>MSLRPCFVSLIDESDKPILIYVPNEAENEMNDVLKYNVLSNISLDYFESALVEWHSLDSKPLLKSIFQLEGVSVFAMLIKQTGLKIVIGFEQKSLSGADDEFEAINQIFETVRKIYIRVKCNPLLVSGDEKSIIKSLERKFDELFISTEVEL[2x];>[2x]MSSTHSNNVGHPQSSPQGPLTEQQRAQQQYQIFENSLPKVSQSVYQMLLNEMVPLAMGIERQISGDVISSDSNVTSENGNINNMIKRLKIEEHHTVDIIRSHNLIHELYKADEEEKEKVLARLRNIGFQIGLKLSELLIFSNNPNLKFKEMDLLLIMKFICRDVWKQIFGKQIDNLKTNHRGTFYLLDYDYRPIQSFSLEEDAKNEELKMIEPFLEIPVGIIRGVLSSLGYSSEEVICLASFIDRPTDRPKTAFPKGVSFHVQVTMPQ;>[4x]MVSTTQSRSLKAMGEEIWKNKTEKINTELFTLTYGSIVAQLCQDYERDFNKVNDHLYSMGYNIGCRLIEDFLARTALPRCENLVKTSEVLSKCAFKIFLNITPNITNWSHNKDTFSLILDENPLADFVELPMDAMKSLWYSNILCGVLKGSLEMVQLDCDVWFVSDILRGDSQTEIKVKLNRILKDEIPIGED;>[2x]MGIYSFWIFDRHCNCIFDREWTLASNSASGTINSKQNEEDAKLLYGMIFSLRSITQKLSKGSVKNDIRSISTGKYRVHTYCTASGLWFVLLSDFKQQSYTQVLQYIYSHIYVKYVSNNLLSPYDFAENENEMRGQGTRKITNRNFISVLESFLAPMVNQ;>[2x]MAIETILVINKSGGLIYQRNFTNDEQKLNSNEYLILASTLHGVFAIASQLTPKALQLTQQTNIENTIPYIPYVGMSSNRSDTRNGGGNNNKHTNNEKLGSFKGDDFFKEPFTNWNKSGLRQLCTDQFTMFIYQTLTGLKFVAISSSVMPQRQPTIATTDKPDRPKSTSNLAIQIADNFLRKVYCLYSDYVMKDPSYSMEMPIRSNLFDEKVKKMVENLQ;>MSQRIIQPSASDQQFPGKSDGYEYTVGPKQAITSEASTTYYISRIYSESLLFKRQEASLSAMAFLFQEMISQLHRTCKTAGDFETKLSDYGHNIGIRLLELLNFRASSSPSSLPRASAFLSQNESSSKLSNASNSPGMLANSSTATSASANERLQEKQTESLSNYITKMRRRDLKILDILQFIHGTLWSYLFNHVSDDLVKSSERDNEYMIVDNFPTLTQFIPGENVSCEYFVCGIIKGFLFNAGFPCGVTAHRMPQGGHSQRTVYLIQFDRQVLDREGLRFG[2x];>[2x]MPQYFAIIGKKDNPVYEIEFTNAENPQGFPQDLKELNPFILHASLDIVEDLQWQINPTSQLNGNGGNGSNGGGGFLRSRAVNNTDNCYLGKVDHFYGLAITAYISYSGMKFVMIHGNSANSSVVIDDNNMRSFYQEVHELYVKTLMNPFYKITDPIRSPAFDSRVRTLARKHLSK;>MDKEIYCGSVPVSYFDPFDLFESLRPEFQQILPLDNIHWKAFDGTVRTVNRLPIELIPEGRGEADKSNDEQPFIRFLIVNCISIDQYRAKVRPLVRQWLPNLESVSSSTGEKMIYKPIILLYANSEVVDSNLFKSVSLMEKFGKDFPHVQTLEVRSVYRSPKERQEFWNQFSQKIKASVLSIFQKRLTHLQHSLANLQKGNNFEEQLLTREKLYELYVVFNILEDASLELQKIKKEILRRNMNMPDGKLQVPFESSSKSDESLGSIIIEGTLDKFQLHKYFFIRRLRLLKLEDQTLTAFVGAFQLIKNFIESISIEYRKSVRLLEFKHYFITSMLSYFEFENVSNPLLCEIKAELLMLKRDNWVQGVMATSGYRLMDKNYPNSDVKYKFDLLKETFVDETVFQENFLTLTKEILSLFNKCEGKRQRIVDILSIEIGLLYYQGKKYEEAVSLFLSCYEYYTQTNWNSIGLKILQVFIDSLSHCPKLDVLQIDGESVSASAVLTNAFLNILKLCKDNDSKEIWWKKFMDLQMKNNIHLMYPLDGLFEVTLNSKVHLARANVSAIEVNLKSYGFPEDISTKTMRLSLKNMGGDVIVFGASDFLLKKGENKLILECRDIMYGEFSLLSFEIIVEGITFVKEFPENQDEFIVVPEIYCKESTKVLVKQAHNLNLGEYALELKSVQSDALESLQVEVEVQKNIGNMKNLPVSFSMDEIQARKRYNTPFENVRLEYYLLDQITAFDLIIKTSFTKKNDQGTFGETKKVRIQCYLQLSVSVEDIFKKDIFFFKFLLNSSVREEPVILYSSELSAPDTRNDYNIRGDYIATTPALITFDGNESFINCYEITANNNFDSKDIFNLKVRYNTLKEQLDCFITDAVLIEGDVEWFILFEKWKTFWELEILKKLKYDYDAFKENRIIRLLKTSIDLNKTKSKIRNLCIEKAVLDKILICLNKVSRGIAVCNTDMDEYVRNLVPKQLTVPVQLPGFEQFFHVQFEQMETSHDALHDTIATIGNSLSYTVIVENLSGQWGQDVIDDGGYIFEILSSNEWLIHGQKRCAIKEKRKEFEVHLIPLKKGYLNFPRVEITNINGKSCRVDHSNAFESILIF[2x];>MNILKHFPSYVGPSKIRTLVIPIGHWTRKEFNNAVQKLSEFNEIHLSDVTPIDSPIFTPQGFPHGKLFFDFLTIDHDDALELFLYDFEPFRKTFVIIGLVNDYSDPLTNLNFMKEKYPTLISPNLVYASSTPTKELEQTIDTMENVFASSPDMQKNIETIMCDIARNFLTALNSYYSSYKHVTLRSPGAIGGNAVLKTTLIRQNSYTSSSSSTPMSAVQSSVSSSSKAGSVTTASKRLSSFEMTTNSLKRSASLKLATTLSTSENRSQQKSLGRQMKILGNFQLLAGRYVDALNSFVDAITTLYKVRDYLWLGSALDGISICFLLLSYLGLSYQIPQIVSLICPVEKLNFESSSTGISPVDSNSKATASTTASSTPRNSISIAAMQSPRNSIMSLSAPALNIDVENINLPLLIKCISDKVLYYYDLSLMHNSEYAPQVVYCEFLLKTLTFMTSCYKSSEFSKDVLDNIVKNQHRALSDIPNSPMFPRFEVYFYSNKLFELQLKEMQVEAQIKIYSTMAEVYRLLGYKRKQLFVLRLLMVALLATPNKIAWHPDYRTLIDTIIELLNINESEAKINVDDPSQSTWLILQKKILQLCIKVSRKINDFEYVAKFSSILITKYTHLLNQSEQDALFKEYIQPSITNESITSYWDPFILREVVINRILDSDPTSNEIPLESDVSSLESLENRQKTQDINPQEVFNPFKRVQPTSFVSNNSTKVPILVFLVGDKAEFTCRVQNPFKFDFTINDIQLDEEISEFCEIDRKAVSYSGPYNVKAESIRSITLPLIIKKPTYKKIYEISCLKISILKLPLQKFDIINDSRRSNPVEEEAEYSKCIYGKLKIKILPEQPQLELLSTSKMTRNSWMMLDGTKTDFHITVRNKSLSCAINHIKIIPMNNIEQMLKPDYWKKMPPDDLYIMEKQLDWLSKSCVRIIKLPTVIKPNETITFDLELDNTAVPFNFTGFDLLIEYGMSATDESCIYLKKLSIPYEVTLRRTIEVPSMDIIPLNELFSSQVENVDWIEYVMSKIRAESNLHSRDFILLLLDFRNSWIDGIKLNVQFEDFTSNEYHVEASHTSRIIVPIKKIDYKKYNFENTPIPRIFPGRQFIQSGLNEEQTIEMRQKFWCREHIISKLKCNWKLTTDQSVTGSVDFNKFIEKFDHKMVYTIYPGRLFYGVQLLLDEPKVKVGEIINLKIITEPTSTCRRKQNSTVNFLDIVIFDSKTSKILPRSNRRILYNGSLTKPISTTKVSEINLEIIPIEKGRYEFSVCISKSNNQDGIIQFDSENVILSVI[2x];>MECFVPLRCDLDGSNIEQLRQSHLSRKFIIFDEQLNLWLWFQGNSQENKRFVLQNMIILINEAQVTRTSTIDDYFTQVENNENLWRLKNDCCSKILFKSNVVMNNGYNNQIKFVFEYKSVDANFNNQDSLQDPQAKYTLDKYSSEEILPSFEPVYSWSSAATKSSKNTNNHLEKNNRATHRVSSKNSEVHEADVSRNPNTFTLKLQYPIFSLLNMRLRNISLKSEH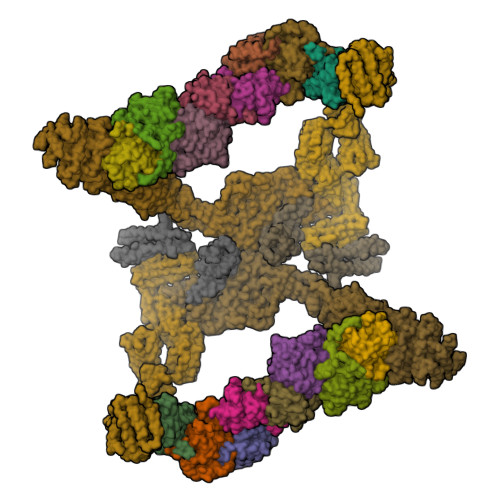CILSSLDFQTSKASEQLTKKFIYPQEHNSFLKLNFQEISYKLIDGTSQIELDPICPLKVPLTAFSYDSISATFKLVLLPKSTQPHRVKITLAYELELHPNLKLPVRTSWETEVTLKRSMPISSTSSQYSSNNNNTNHSASFNGAANNVNSGGLANLRLGGVSSSRFSLGAASTTSLVNSKLSNVKFKFINSNIKVIKGEKFTMRLQIINSSSSPLDLVVYYNNTINPIPSANNVRNSNGINNCGMNNGTIPNSPLTLENQYQLHNKYRKIAEGIILLSNDYKIPVVPPRETYFADLRFIGIMSGYYGTLSGLKVLDLNTNELIEVGNGASVLIQ[2x]> MNELPIILLSPLIGGALAWLIRVKGIREAIGVVSSAIPLYFLIKLYPALEGEPIRYSLNVGGFELT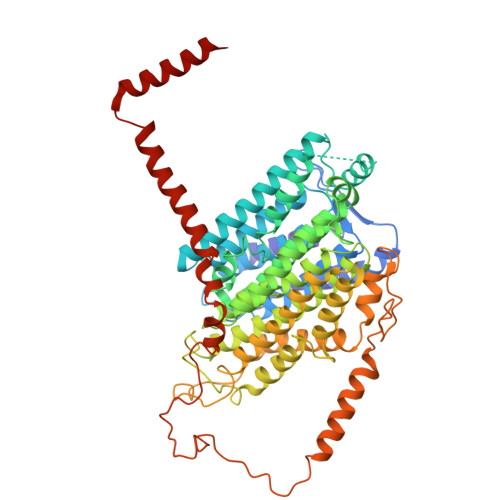LALSHISWIFAMIAAVVGLSAVLGLVSTAKDSNEWLFALMSLAGALGVFLANDFVVFFLSWEIMTFASFMMVFKYNRHASLKYFVLSIAGAYAMLLAIGIIYAKTGSLSFPEISAIFRQDAMMGMMGGGGVFTKTETLLIYALFLVAFGVKAGMFPLHVWAPDAYSETNQSYTAMFSGVLSKTGVYGFFLLYLLMYGKLAITLGNVRSAPTFGYIIAFLGGLTIMVGGILAALQEDIRKLFAYSSISQIGYILIGLGIGTPLGIAAATYHAISHALFKGLFFLIVATIIYRTGKTEFKDYGGLAEKMPITFAMAFVAILSLAGIPPMAGFASKWLIFEAVISRNLPILGAMVFFGSAIGFVYLIRFTYAVWFGQRPSDLEDVKDAPLPLAIGMGILAILNVIFGVAPGLVARELNKLFSNPPIGGTIWELDLGFGRYNGLLLSIWLVIGLIIAAILYFMGAGVRKVPVTDTYQSGNPVTMEYNLTIRRNFFLPLKEAMAFWLKMSFDRLYHDIWKAIEELADLARSYVYNGNIQAYAWYLAIILLILVAMGV>[2x]MASWSHPQFEKMGMLEARELLCERDERTLFSGLSFTLNAGEWVQITGSNGAGKTTLLRLLTGLSRPDAGEVLWQGQPLHQVRDSYHQNLLWIGHQPGIKTRLTALENLHFYHRDGDTAQCLEALAQAGLAGFEDIPVNQLSAGQQRRVALARLWLTRATLWILDEPFTAIDVNGVDRLTQRMAQHTEQGGIVILTTHQPLNVAESKIRRISLTQTRAA;>MMFWRIFRLELRVAFRHSAEIANPLWFFLIVITLFPLSIGPEPQLLARIAPGIIWVAALLSSLLALERLFRDDLQDGSLEQLMLLPLPLPAVVLAKVMAHWMVTGLPLLILSPLVAMLLGMDVYGWQVMALTLLLGTPTLGFLGAPGVALTVGLKRGGVLLSILVLPLTIPLLIFATAAMDAASMHLPVDGYLAILGALLAGTATLSPFATAAALRISIQ[2x];>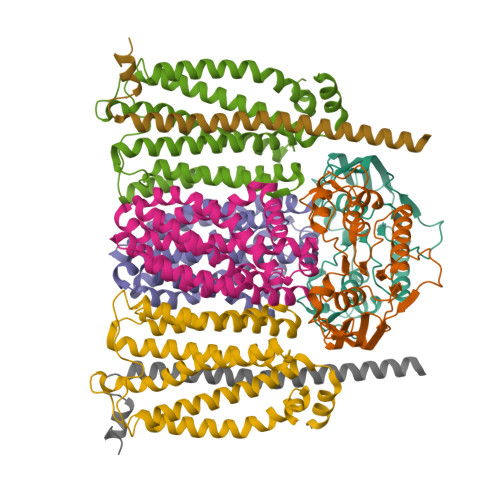MWKTLHQLAIPPRLYQICGWFIPWLAIASVVVLTVGWIWGFGFAPADYQQGNSYRIIYLHVPAAIWSMGIYASMAVAAFIGLVWQMKMANLAVAAMAPIGAVFTFIALVTGSAWGKPMWGTWWVWDARLTSELVLLFLYVGVIALWHAFDDRRLAGRAAGILVLIGVVNLPIIHYSVEWWNTLHQGSTRMQQSIDPAMRSPLRWSIFGFLLLSATLTLMRMRNLILLMEKRRPWVSELILKRGRK[2x];>MTPAFASWNEFFAMGGYAFFVWLAVVMTVIPLVVLVVHSVMQHRAILRGVAQQRAREARLRAAQQQEAA[2x]>[2x]MSTPAPPEEQARLLEDALIAVRQQTAMMRKFLDTPGKLMDALKCCSTLVSELRTSSLSPKQYYELYMAVFDALRYLSAHLRENHPVNHLADLYELVQYAGNIIPRLYLMITVGTAYMSIDGAPVKELMKDMMDMSRGVQHPVRGLFLRYYLSGQARDYLPTGDSDGPEGNLQDSINFILTNFVEMNKLWVRLQHQGHSRERDLRTQERRELQLLVGSNIVRLSQLVDLPTYRDSILGPLLEQIVQCRDILAQEYLLEVITQVFPDEYHLHTLDQFLGAVSRLNPHVN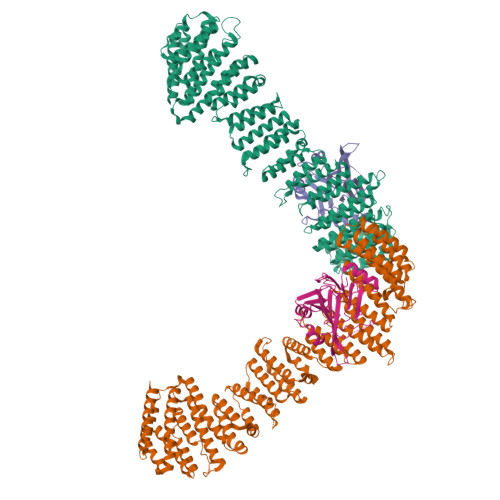VKAIVIGMMNRLSDYAERESQNEPEEDRAKLEEEALAKLLEKTKLGQNSELEPQNGDHPDTEVSSTTDSAQAPSTADSDTTAVNGEEEPVRKRRGIPVNVPLYDIFFDQVQHLVQAQHLPIQDTIALCCSLANLSLNIYPERLDYVDGILAYALAKVKEHANSADLHSQPAQQSLLSLLQSPLRRYVSIFTALSLPTYVSLFQAQTYPTRRAIAGEIVRTLLKNQTLISTPAHLENVLEILKVLIKEGSQPPAGYPGVVQPRARPLETDETMEEQGWLARLVHLIHSDDNDTQFRLLQMTRKAYAEGNERIRTTTPPLITAGLKLARRFKAREHYDDNWSSQSSSLFKFLHSAISTLYTRVNGPGVADLCLRLFCSCGQVADMTEFEEVAYEFFAQAFTVYEESISDSKAQFQAVCVIASALHRTRNFGRENYDTLITKCAQHASKLLRKPDQCRAVYLASHLWWATPIAARGETEDTELYRDGKRVLECLQRALRVADSCMETATSIELFVEILDRYVYYFDQRNESVTTKYLNGLIELIHSNLAGNQQDSASVEASRKHFIQTLEMIQSKEFEGIVVAPK;>[2x]SMAFLILVIGNLHIPDRALDIPPKFKKLLSPGKISQTLCLGNLTDRATYDYLRSISPDLKIVRGRMDVEATSLPLMQVVTHGSLRIGFLEGFTLVSEEPDVLLAEANKLDVDVLCWAGGSHRFECFEYMDKFFVNPGSATGAFTTDWLAEGEEVVPSFCLMDVQGISLTLYVYQLRKDENGTENVAVEKVTYTKPVEPTGAS> MPEVVFGSVTDLGYAAGWRLVRAMPEAMAQGVFGAGARYAARNGGPEQLRRNLARVVGKPPADVPDDLIRASLASYARYWREAFRLPAMDHGRLGEQLDVIDIDHLWSALDAGRGAVLALPHSGNWDMAGVWLVQNYGPFTTVAERLKPESLYRRFVEYRESLGFEVLPLTGGERPPFEVLAERLTDNRPICLMAERDLTRSGVQVDFFGEATRMPAGPAKLAIETGAALFPVHCWFEGDGWGMRVYPELDTSSGDVTAITQALADRFAANIATYPADWHMLQPQWIADLSDERRARLGTSRHHHHHH

Here, X-ray crystallography, site-directed mutagenesis and enzymatic activity data are used to define the three-dimensional structure, acceptor/donor substrate binding, membrane binding and catalytic mechanism of PatA from M. smegmatis. PatA catalyses an essential step in the biosynthesis of PIMs in M. tuberculosis. The enzyme transfers a palmitoyl moiety from palmitoyl–CoA to the 6-position of the Manp ring linked to 2-position of myo-inositol in PIM1 or PIM2. Our results reveal that the enzyme has an α/β architecture and shares with other important eukaryotic/prokaryotic acyltransferases an acid/base catalytic mechanism involving conserved histidine and aspartic/glutamic acid residues.

Two other crystal forms were obtained in P 21 (PatA–C16-2) and P 42212 (PatA–C16-3) space groups, and the corresponding crystal structures solved at 2.90 and 2.43 Å resolution, respectively, by using molecular replacement methods. The high quality of the electron density maps allowed the trace of residues 41 to 302 (PatA–C16-1), 48 to 295 (PatA–C16-2) and 48 to 303 (PatA–C16-3). We have decided to use the PatA–C16-1 crystal form for our description since it displays the highest resolution. A close inspection of the three crystal structures revealed that the protein crystallized as a monomer, displaying a high degree of structural flexibility in the N- and C-terminal regions (coloured in green in Supplementary Fig. 3; root-mean-square deviation (r.m.s.d.) value of 1.6 and 8.4 Å for Cα atoms in 41–47 and 288–302 residue ranges for the N and C terminus, respectively). Strikingly, one molecule of palmitic acid was unambiguously identified in the difference electron density maps of PatA–C16-1, PatA–C16-2 and PatA–C16-3 crystal structures. We believe that acyl molecule is associated to the enzyme due to the hydrolysis of palmitoyl–CoA during the isolation and purification of PatA from M. smegmatis mc2155. The acyl chain is deeply buried into the hydrophobic pocket, and oriented with the carboxylate group facing the groove and the acyl tail extending into the globular core of the monomer. Interestingly, the comparison of the three crystal structures revealed conformational flexibility in the carboxylate moiety of the palmitate, located in close proximity with the lateral chain of H126. In all crystal structures of palmitoyl–PatA and PatA–S-C16CoA complexes, the carboxylate OE2 oxygen atom of E200 was found at 2.8 Å of the ND1 nitrogen atom of the aromatic imidazole ring of the invariant H126. It is worth noting that when the individual palmitate molecules observed in the three crystal structures of palmitoyl–PatA were superimposed, they showed important structural flexibility at the carboxylate region, suggesting that the carboxylate group is not in a catalytically competent position in the crystal structures.> MGAQVSTQKTGAHETGLNASGNSIIHYTNINYYKDAASNSATRQDFAQDPGKFTEPVKDIMIKSLPA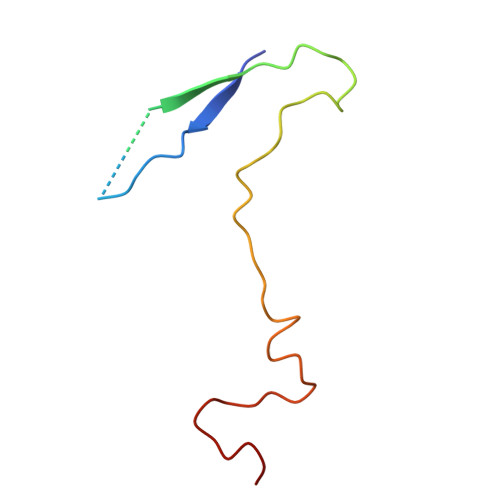LN>[2x]MHHHHHHENLYFQGADESFNLWQECATRCTLDLAQGVRASQLDVASLLGEQAGSGVLHYSMVLEEGGDSLKLALGNALTLRTDGTTITLTSATAGKGPRTYSYTRQGRGNWSLHWLVPVGDDAPASIKVFFHELDAGSEVSHISPIYSIEVSDDLLRTMASNSTLFVRHVENNEINRSLTLSAAGVGFVAAPTQHSRQKRWSEWHTGKVLCLLDPLDAVYNYLSQRTCNLGDTWEGKVYRVLAGTPASHDTHIVPTAISHRLHFAKGDGLAALTTHQVCAIPLESLARSRQPRGWEELSQCGYPVHNLVTLYLLTRLPWSQLDTVITQALANTTPEDGSTPRGQLAQAIRENPAQARLALSMAAAQSDAFSHQQAGNSQEQAASADVVNLTCPAADLNCLAPADSADALQERDYPNGASFLGDGDEVSFSTAGTRNWSVTRLEQAHRQLLARGYLFVGYHGTFLEAAHSIVFEGVHERDQSSIAPWQGFYVAGDPALAYGYAQDQEADARGRIRNGVLLRVYVPRAALPRLFATQQTLAAPGAVDEIGRLIGHPLPLQLEAITGPEEEGGRLATILGWRLAEQAVVIPSTIPTDPRNVGGDLDPASVPQEESAISTLPDYTTQPRDEL

Members of the diphthamide-specific class of mono-ADP-ribosyl transferases (mART), which include the diphtheria toxin (DT), Pseudomonas exotoxin A (PE) and Vibrio cholerae cholix (Chx), are potent bacterial toxins that specifically modify the diphthamide residue of eukaryotic ribosomal elongation factor 2 (eEF2), which plays an essential role in protein synthesis. These toxins catalyse the transfer of ADP-ribose from nicotinamide adenine dinucleotide (NAD+) onto the diphthamide, which results in inhibition of protein synthesis and thus death of the host eukaryotic cells. Among the many virulence factors produced by Aeromonas, a Pseudomonas exotoxin A homologue, AE, was shown to be expressed and play a key role in the virulence of Aeromonas hydrophila strains causing necrotising fasciitis, likely by causing tissue damage. The tri-domain crystal structure provides strong evidence that AE is a fourth member of this toxin family.

The crystal structure of AE was solved at 2.3 Å and presents a three-domain fold similar to other diphthamide-specific mART toxins. Recombinant AE produced here was a catalytically inactive mutant E571A, corresponding to residues 13–626 of the full-length toxin. AE crystallised in the P1211 space group with two identical molecules per asymmetric unit (rmsd of 0.62Å over 601 Cα atoms). Overall, the structure of AE presents a tri-domain architecture similar to PE and cholix with root-mean-square deviation (rmsd) of 2.5 and 2.9 Å, respectively, and includes 4 strictly conserved disulphide bridges. Importantly, this domain holds a furin protease recognition site identical to the one in PE, corresponding to sequence RQPR, with the scissile bond between R291 and G292. In the substrate-free AE structure presented here, loop 1 takes on an intermediate position, which sees the main chain of R476 and Q478 in relatively similar location to their equivalent in the NAD+-bound PE structure, with the glutamine side group within hydrogen bond distance of the adenine-phosphate. On the other side, a deep negatively charged cavity formed between domains II and III leads to a central interdomain interface and reveals a potential metal binding site. No strong anomalous signal was observed for the metal ion in the electron density map, and without any obvious metal source from the crystallisation conditions, structure refinement showed a Na+ ion was the best fit. The bound ion presents a tetrahedral coordination mediated by residues from the three different domains: E409 (domain Ib), H274 (domain II), E471 (domain III) and a water molecule stabilised by D411. It should be noted that although AE was crystallised at pH 5.5, it presents an overall fold similar to the structures of PE and Cholix, which were solved at pH 7.5–8.0.UBR4 is a 574 kDa E3 ligase (E3) of the N-degron pathway with roles in neurodevelopment, age-associated muscular atrophy and cancer. Here we identify and characterize a distinct E3 module within human UBR4 consisting of a ‘hemiRING’ zinc finger, a helical-rich UBR zinc-finger interacting (UZI) subdomain, and an N-terminal region that can serve as an affinity factor for the E2 conjugating enzyme (E2). Via an allosteric mechanism, the UZI subdomain modestly activates the Ub-loaded E2 (E2∼Ub).

To determine the structure of this complex, we obtained crystals and collected diffraction data to 3.2 Å. A structure was solved by molecular replacement using the apo structure obtained from UBR4xtal, and a UBE2A crystal structure. As for the apo structure, the N-terminal ∼100 residues in the UBR4xtal construct were unresolved. The UBR4 molecule was equivalent to the apo structure (RMSD of 0.98 Å), except for the hemiRING loop connecting αA and αB, gaining structural order, suggestive of E2 binding having a stabilizing effect. Two UBE2A molecules are present in the asymmetric unit, where the first E2 molecule (UBE2A #1) binds the hemiRING proximal to the zinc coordinating fold, as observed with RING domains. Several X-linked intellectual disability (XLID) patient mutations within UBE2A cluster at this interface. Thus, the UBE2A #2 interaction is probably a consequence of crystallographic packing. The most notable interactions arise from UBE2A residues Arg7, Arg8, Arg11, Arg95 and Ser97. The guanidino groups of Arg7 and Arg11 hydrogen bond with the side chain of UBR4 Glu4843. UBE2A Ser97 side chain also forms an important anchor point by hydrogen bonding to the backbone carbonyl of UBR4 Ile4840, the side chain of which also makes hydrophobic contacts with UBE2A Pro98.

> GPLGSAIQHPGTQVLIGTDSIPNLHKLEQVSSDEGIGTLAENLLEALREHPDVNKKIDAARRETRAEKKRMAMAMRQKALGTLGMTTNEKGQVVTKTALLKQMEELIEEPGLTCCICREGYKFQPTKVLGIYTFTKRVALEELENKPRKQQGYSTVSHFNIVHYDCHLAAVRLARGREEWESAALQNANTKCNGLLPVWGPHVPESAFATCLARHNTYLQECTGQREPTYQLNIHDIKLLFLRFAMEQSFSADTGGGGRESNIHLIPYIIHTVLYVLNTTRATSREEKNLQGFLEQPKEKWVESAFEVDGPYYFTVLALHILPPEQWRATRVEILRRLLVTSQARAVAPGGATRLTDKAVKDYSAYRSSLLFWALVDLIYNMFKKVPTSNTEGGWSCSLAEYIRHNDMPIYEAADKALKTFQEEFMPVETFSEFLDVAGLLSEITDPESFLKDLLNSVP;>[2x]GHMLGSMSTPARRRLMRDFKRLQEDPPAGVSGAPSENNIMVWNAVIFGPEGTPFEDGTFKLTIEFTEEYPNKPPTVRFVSKMFHPNVYADGSIKLDILQNRWSPTYDVSSILTSIQSLLDEPNPNSPANSQAAQLYQENKREYEKRVSAIVEQSWRDC(1R,2S,3S,4S,5R,6R)-6-(HYDROXYMETHYL)CYCLOHEXANE-1,2,3,4,5-PENTOL | C7 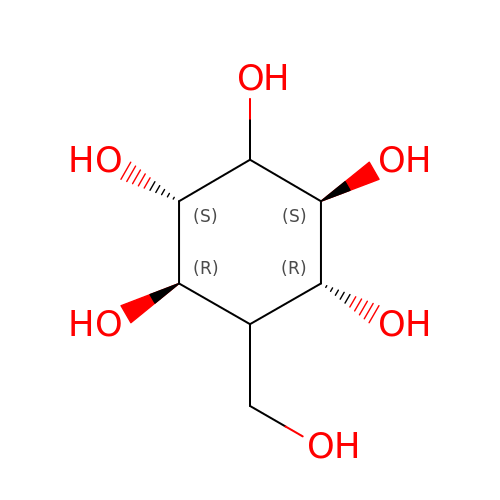H14 O6 | QFYQIWDMMSKNFF-NYLBLOMBSA-N> MKKEVRKVRIALASPEKIRSWSYGEVEKPETINYRTLKPERDGLFDERIFGPIKDYECACGKYKRQRFEGKVCERCGVEVTKSIVRRYRMGHIELATPAAHIWFVKDVPSKIGTLLDLSATELEQVLYFSKYIVLDPKGAILNGVPVEKRQLLTDEEYRELRYGKQETYPLPPGVDALVKDGEEVVKGQELAPGVVSRLDGVALYRFPRRVRVEYVKKERAGLRLPLAAWVEKEAYKPGEILAEL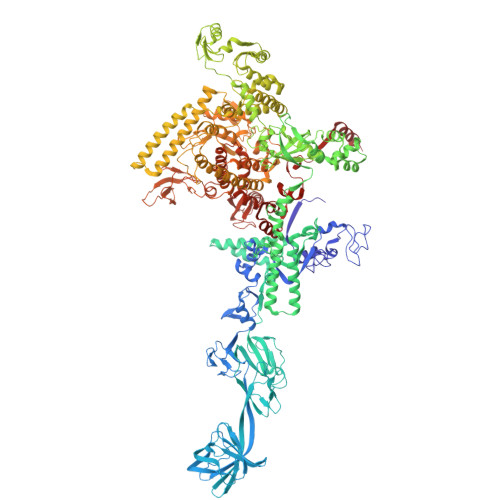PEPYLFRAEEEGVVELKELEEGAFLVLRREDEPVATYFLPVGMTPLVVHGEIVEKGQPLAEAKGLLRMPRQVRAAQVEAEEEGETVYLTLFLEWTEPKDYRVQPHMNVVVPEGARVEAGDKIVAAIDPEEEVIAEAEGVVHLHEPASILVVKARVYPFEDDVEVSTGDRVAPGDVLADGGKVKSDVYGRVEVDLVRNVVRVVESYDIDARMGAEAIQQLLKELDLEALEKELLEEMKHPSRARRAKARKRLEVVRAFLDSGNRPEWMILEAVPVLPPDLRPMVQVDGGRFATSDLNDLYRRLINRNNRLKKLLAQGAPEIIIRNEKRMLQEAVDALLDNGRRGAPVTNPGSDRPLRSLTDILSGKQGRFRQNLLGKRVDYSGRSVIVVGPQLKLHQCGLPKRMALELFKPFLLKKMEEKGIAPNVKAARRMLERQRDIKDEVWDALEEVIHGKVVLLNRAPTLHRLGIQAFQPVLVEGQSIQLHPLVCEAFNADFDGDQMAVHVPLSSFAQAEARIQMLSAHNLLSPASGEPLAKPSRDIILGLYYITQVRKEKKGAGLEFATPEEALAAHERGEVALNAPIKVAGRETSVGRLKYVFANPDEALLAVAHGIVDLQDVVTVRYMGKRLETSPGRILFARIVAEAVEDEKVAWELIQLDVPQEKNSLKDLVYQAFLRLGMEKTARLLDALKYYGFTFSTTSGITIGIDDAVIPEEKKQYLEEADRKLLQIEQAYEMGFLTDRERYDQILQLWTETTEKVTQAVFKNFEENYPFNPLYVMAQSGARGNPQQIRQLCGLRGLMQKPSGETFEVPVRSSFREGLTVLEYFISSHGARKGGADTALRTADSGYLTRKLVDVTHEIVVREADCGTTNYISVPLFQPDEVTRSLRLRKRADIEAGLYGRVLAREVEVLGVRLEEGRYLSMDDVHLLIKAAEAGEIQEVPVRSPLTCQTRYGVCQKCYGYDLSMARPVSIGEAVGIVAAQSIGEPGTQLTMRTFHTGGVAGAADITQGLPRVIELFEARRPKAKAVISEIDGVVRIEETEEKLSVFVESEGFSKEYKLPKEARLLVKDGDYVEAGQPLTRGAIDPHQLLEAKGPEAVERYLVEEIQKVYRAQGVKLHDKHIEIVVRQMMKYVEVTDPGDSRLLEGQVLEKWDVEALNERLIAEGKTPVAWKPLLMGVTKSALSTKSWLSAASFQNTTHVLTEAAIAGKKDELIGLKENVILGRLIPAGTGSDFVRFTQVVDQKTLKAIEEARKEA Our subsequent work demonstrated that the HEPN protein with a RX4–6H motif is the toxin which cleaves mRNA in vitro in the HEPN/MNT (SO_3166/SO_3165) TA pair in the model psychrotrophic bacterium Shewanella oneidensis. Furthermore, antitoxin SO_3165 binds to toxin SO_3166 at a rare 2:6 ratio to form a hetero-octamer, and this binding is important for the antitoxin to block the toxicity of the toxin. Specifically, structural and biochemical studies of the HepT/MntA TA pair (SO_3166/SO_3165) in S. oneidensis show that the GSX10DXD motif of antitoxin MntA is responsible for transferring three AMPs to HepT and that Y104 in RX4HXY in HepT is the site that receives three AMPs from MntA. We found here that MntA antitoxin acts as an adenylyltransferase and catalyzes the transfer of three AMP moieties onto toxin HepT to block its toxicity, representing a new type of interaction between the toxin and the antitoxin.

We determined the crystal structures of HepT/MntA and HepTY104A/MntA at 3.08 and 2.6 Å, respectively. There were four molecules composed of one MntA polypeptide and three HepT polypeptides in one asymmetric unit (ASU), and the complex formed a hetero-octamer based on symmetry analysis; this result is consistent with our previous report. During structure determination, three regions of the unambiguous electron map connected to the hydroxyl group of Y104 in HepT were exclusively observed in the structure of WT HepT/MntA. In view of the above mentioned results, antitoxin MntA polyadenylylates toxin HepT, and in the final structure, a total of three AMP moieties linked by 3′-5′ phosphodiester bonds were accommodated in every region of the additional electron density map. Y104 of HepT was polyadenylylated, and a phosphodiester bond was formed by the α-phosphate of the first AMP (AMP1) and the hydroxyl group of Y104. Interestingly, detailed analysis of the AMP triplet moieties of the three HepT molecules in the ASU revealed that the orientation on Chains A or B was different from the one on Chain C. For clarity, the polyadenylylated structures of chain A of HepT and chain C of HepT were extracted. The AMP moiety in Chain A was twisted toward the cleft formed by α4 and α5 of HepT. In contrast, the AMP moieties in chain C of HepT were oriented to MntA. The analysis of the interaction of HepT and the AMP moieties revealed that AMP fits near the cavities along the cleft access to the RX4H RNase activity site. Furthermore, the highly conserved R70 that was located in the positively charged region of HepT forms hydrogen bonds with the first AMP moiety.

> MQQLNENKIIKLLRDNIPKLQLIYLFGSYSQGTQHRNSDIDIAVLAADTLDNIARWELAQKLASALDSDVDLVDLRSASTVLCQQVVTQGKQLWGTQQDDELFAVKTISMYQHLQAERQAIIDDVMANTAAKAHRGESL;>MNDIIINKIATIKRCIKRIQQVYGDGSQFKQDFTLQDSVILNLQRCCEACIDIANHINRQQQLGIPQSSRDSFTLLAQNNLITQPLSDNLKKMVGLRNIAVHDYQELNLDIVVHVVQHHLEDFEQFIDVIKAE[3x]> MKEQLEDVLDTLTDREENVLRLRFGLDDGRTRTLEEVGKVFGVTRERIRQIEAKALRKL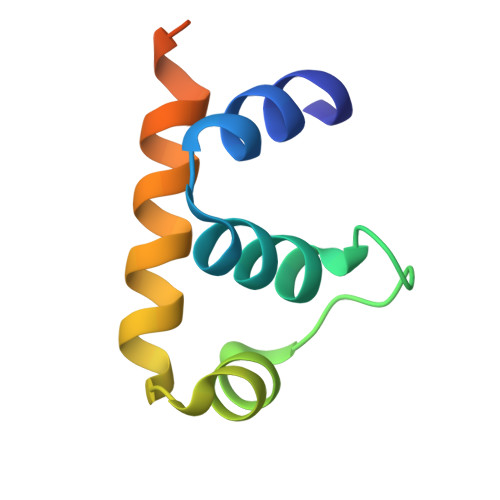RHPSRSKRLKDFMD>MEASPASGPRHLMDPHIFTSNFNNGIGRHKTYLCYEVERLDNGTSVKMDQHRGFLHNQAKNLLCGFYGRHAALRFLDLVPSLQLDPAQIYRVTWFISWSPCFSWGCAGEVRAFLQENTHVRLRIFAARIYDYDPLYKEALQMLRDAGAQVSIMTYDEFKHCWDTFVDHQGCPFQPWDGLDEHSQALSGRLRAILQNQGN[2x]

The APOBEC3 family of enzymes (A3A-A3H) forms part of the innate immune response against viruses and transposons. The normally antiviral enzyme APOBEC3A is an endogenous mutagen in human cancer. Its single-stranded DNA C-to-U editing activity results in multiple mutagenic outcomes including signature single-base substitution mutations (isolated and clustered), DNA breakage, and larger-scale chromosomal aberrations. Here, we use X-ray crystallography to determine high-resolution structures of wildtype A3A/hairpin-inhibited complexes and demonstrate the underlying mechanism of inhibition.

Surprisingly, they also share very similar conformation of the hairpin loop region’s TT(C/FdZ)G moiety. The superpositions of A3A-E72A in complex with the 3-nt loop, TTC-hairpin (at 2.22 Å resolution), and the 4-nucleotide loops, ATTC-hairpin (at 1.91 Å resolution) and CTTC-hairpin (at 3.15 Å resolution), are mostly similar with an average RMSD of 0.43 Å (ribbon schematics in Fig. 2b and Supplementary Fig. S3c). Larger 4-nt loops extrude one nucleotide to optimally fit around the A3A active site. First, His29 base-stacks with G+1, and T−2 base-stacks with a pyrimidine in the stem (C−3 for the 3-residue loop or C−4 for the 4-residue loop). Second, the positively charged guanidinium moiety of Arg28 forms a cation-π interaction with the nucleobase T−2, thereby further stabilizing T−2 placement for interaction with His29. Arg28 also forms a hydrogen bond to an oxygen atom of the phosphate linking A−3/C−3 to T−2, and the cytosine at position −4 is in register to hydrogen bond with guanine at position +1 as a part of hairpin’s stem. Third, the tight turn between the nucleotide at position +1 and the target cytosine at position 0 is stabilized by a bifurcated hydrogen bond between Nδ1 (amine tautomer) of His29 and O4′ of 2-deoxyribose at +1 and an oxygen atom of the phosphate group that links nucleotides C0 and T−1. Last, the peptide NH group of Lys60 hydrogen bonds to the phosphate linking nucleotides at positions 0 and +1, and the -NH3+ moiety of its side chain forms a salt bridge to the phosphate group linking nts +1 and +2. Our structural studies establish that the stem-loop preconfigures the primary TC recognition motif in optimal position for binding to A3A, such that hairpin DNAs are more reactive substrates and as the 2′-deoxy-5-fluorozebularine derivative is a more potent inhibitor of A3A than linear ssDNA. Both 3- and 4-nt loops present the TC or TTFdZ motif in an identical configuration to A3A.Here we report that the 2-aminoisobutyric acid hydroxylase from Rhodococcus wratislaviensis, AibH1H2, requires manganese to functionalize a strong, aliphatic C–H bond (BDE = 100 kcal/mol). Structural and spectroscopic studies of this enzyme reveal a redox-active, heterobimetallic manganese–iron active site at the locus of O2 activation and substrate coordination. Metabolism of 2-aminoisobutyric acid (AIB) in Rhodococcus wratislaviensis proceeds via the initial, selective hydroxylation of the pro-(R) methyl group by the monooxygenase AibH1H2 to furnish α-methyl-d-serine (d-MeSer). Previously, recombinant expression of AibH1H2 in Escherichia coli enabled its structural characterization and revealed distinct mono- and dinuclear metal binding sites housed within the AibH1 and AibH2 protein subunits, respectively.

We expressed AibH1H2 in E. coli grown in M9 minimal medium supplemented with excess FeII, and subsequent purification furnished protein samples (FeAibH1H2) containing ∼3 equiv of Fe per AibH1H2 heterodimer and minimal heterometal content (entry 1). Fe occupancy in both the mononuclear (Site 0) and dinuclear (Sites 1 and 2) metal sites was evident by inspection of the anomalous dispersion maps obtained from X-ray diffraction experiments performed on single crystals of FeAibH1H2. AibH1H2 had no detectable activity upon the exclusive incorporation of iron ions. To probe whether the absence of monooxygenase activity was caused by the choice of sacrificial reductant, other commonly utilized reducing systems (e.g., NADH/Phenazine, sodium dithionite, and alpha-ketoglutarate) were explored, but none proved competent to produce measurable quantities of d-MeSer with FeAibH1H2. These results suggested that the active form of AibH1H2 could not be produced under routine expression and purification conditions typically used for nonheme iron enzymes.

>[2x]MGHHHHHHSGENLYFQSGGMVAPTSNPGVPDELDGVPAVVDCDVHAVLPSPHSLIPYLDEYWADQLVAQLAPTYEPNYHPRGSAIAQHSDASVDENGRAATTAENLVKDVFADGFTDFAVVNCLYGVQQIHQPRREMAHARALNHWIANEWLDKDDRLRASIVVPQGSPRAAAEEIDFWSGDKRFVQVLLLGQSELLYGREINWPIWEAAEAAGLPVTLHIGGVFRQAPTSVGWPASHLEWYVGQQSNIEAQLNSIISEGILQKFPKTKILLSELGFNWLPPFMWKFDKLWKSYRPDIPWVQESPLELIREHVRVTTSPSDGAEEAGRLDSIVDRLGSDRMLVYSSDYPHKHHSGPRDIENGTHSPELLDRIYRRNAFDLYNLVVPSPGKVG;>MTIIEHGSLGTLPAPSVTTGIVDADIHPVPQDGALEPYLDDRWKKHIREYGVRTTTGLQFISEYPQMYGGAMRADAWPESGYPGSDRELLRTQLLDKHNIQLGVLQCLAPGGQTLNPAGQALNQELAAALCRATNDWQLEHLVYPDPRMRAAIPVTFETPDYAVAEIERVGADPGVVAVLGTSKTLEPLGSRKYWPIYEASVAQNLPIQFHLSQGGGHANTGTGWTSYHTEYHTGHVQSFQSQLLSLVLSGTFDRFPTLKVMFVEGNVAHFAPLIQRMDYTWETLRGELPDLQRKPSEYIRDHIWASTQPIDEPEKPEHLAELLEEFCGDNVVFATDYPHFDFDDPETAFPRSFPVDLRDKILRGNGMRFFGVTNQAD[2x]>[2x]SNAMLKGKYTK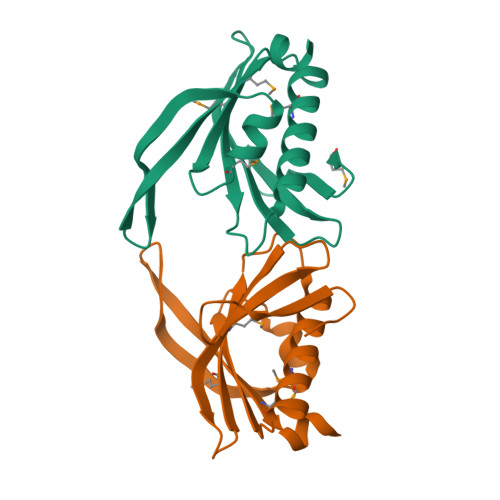IEKVNGVEREYLITDKYGITIGRIFIVDLNKDNRFCMFRMKIYKQGKSINTYIKEILSVFMEFLFKSNDINKVNIIVDEEVSTQPFVELGFAFEGIINKSIIEKNVLKDEFLFGMDYKNYNSDR β‐1,2‐Glucans are natural glucose polymers produced by bacteria and play important physiological roles, including as symbiotic or pathogenic factors and in osmoregulation. Glycoside hydrolase (GH) families related to β‐1,2‐glucan metabolism (GH144, GH162, and GH189) have recently been created by identification of two β‐1,2‐glucanases and a β‐1,2‐glucanotransferase, respectively. Structural analysis of the proteins in Groups 1–4 revealed that they possess (α/α)6‐barrel folds similar to those of GH144, GH162, and GH189 enzymes. Overall, phylogenetic, biochemical, and structural analyses revealed that Groups 1–3 are new GH families, GH192, GH193, and GH194, respectively, and that the three families belong to clan GH‐S (clan GH, classification based on structural similarity) as GH144 and GH162.

In this study, we used PgSGL1, PgSGL2 from Photobacterium gaetbulicola and EeSGL1 from Endozoicomonas elysicola as Group 1 proteins; SkSGL from Sanguibacter keddieii, a Gram‐positive bacterium, as a Group 2 protein; PgSGL3 and PgSGL4 from P. gaetbulicola as Groups 3 and 4 proteins, respectively. Groups 1 and 3 contained proteins from many marine bacteria, for example, isolated from marine sediment and mudflat environments. Because hydrolytic activities toward β‐1,2‐glucans were detected for PgSGL1, PgSGL2, PgSGL3, EeSGL1, SkSGLc, and XcSGL, the general properties of these enzymes were investigated using β‐1,2‐glucan alditols (see Section 4 for details) as substrates. While many of the enzymes showed optimal pH values around neutral pH, the optimal pH values of PgSGL3 and XcSGL were 8.5 and 5.0, respectively, which suggests that the optimal pH value varied within the SGL clan. PgSGL1 and PgSGL3, single‐domain enzymes, were eluted at the time corresponding to 42 kDa, while the elution time of SkSGLc corresponded to 140 kDa. These results indicated that PgSGL1 and PgSGL3 were monomeric enzymes and SkSGL was a dimeric enzyme. Interestingly, PgSGL3 (Group 3) produced Sop8 predominantly in the initial stage of the reaction, and then Sop8 was further hydrolyzed (left). When Sop8 was used as a substrate, Sop8 was hydrolyzed to Sop3–5 (right). The five enzymes (Groups 1–3) were clearly identified as SGLs.

> MQTAANDTVISETVKSDQEIIDSLYRGGYAYWQQLRNENGTYEDKLFLNGDRSYVGSIANSGMGLIALTIGHANGWEPEAEQLALVTLRKLAGRDPNFAVPQNATNTFIHFYNTKTGEAVGDDWSPVDSAIMIYGALFVKNYFSENEEIAELADFLYRNTDLTQYIADVRTGRIYLAQHTDGTFKKYRTKAFNEYMLVAGIANQQAKDLDNAVNASNAKKFWDIWYASTKFLPVAEYNGIPVLSEGKTWFTSQFNFLFNNYLMHDFSNHPEFVTALENSAKADFAFWRDVDVEGVELKEYEWGSGAGSCPNGYCVDRFHFDGDRQFNHNLVVSPHILAGYIPFNDRAKADLISTYRDNTINAKHELEGGYEILWRYSHDQPEWKAEFIEGVDFSTFLFGLAAMPEHLGMDFFNKYNNYFELEHHHHHH>GSDGGTLAMLRGLSEDTLEQLYALGFNQYQAGKWDDAQKIFQALCMLDHYDARYFLGLGACRQSLGLYEQALQSYSYGALMDINEPRFPFHAAECHLQLGDLDGAESGFYSARALAAAQPAHEALAARA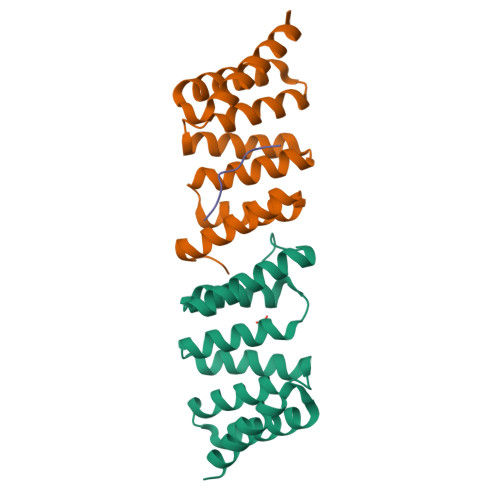GAMLEAVTARKDR[2x];> DRVELNAPRQ>[4x]VRYRFLRLAPDEEGEGGRAESRILECRRLRAPAEIARALELRAGETVVTIRRQLSMNHMPTVIDDLWLPGTHFRGLTLELLTASKAPLYGLFESEFGVSMVRADEKLRAVAA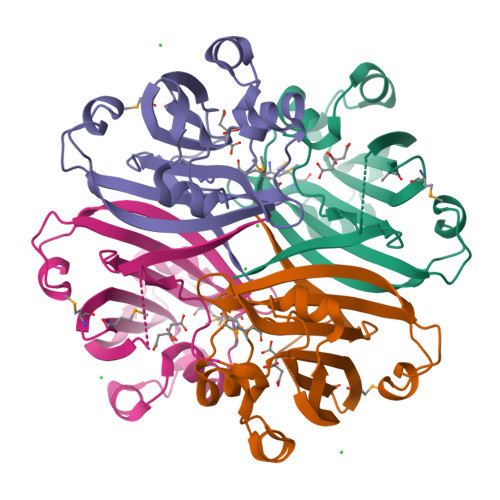SPEIAPLLGVEPGRPLLQVDRISYTYGDRPMEVRRGLYLTDHYHYRNSLN> CPLHWSSYNGYCYRVFSELKTWEDAESFCYAQHKGSRLASIHSREEEA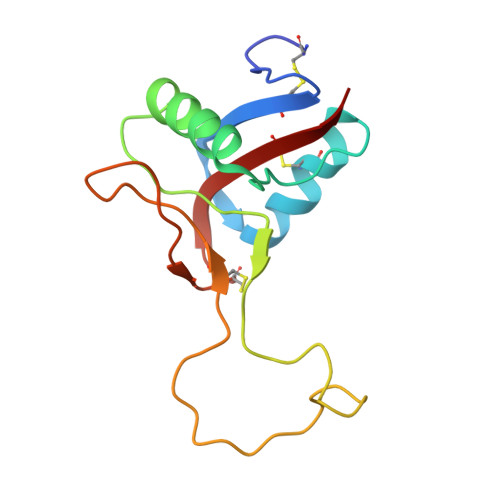FVGKLASQTLKYTSMWLGLNNAWAACKWEWSDDAKLDYKVWLRRAYCAVMVVKTDRIFWYNRGCEKTVSFLCKFYS> MLPKDKLNPPTPSIYLENKRDAFFPPLHQFCTNPKNPVTVIRG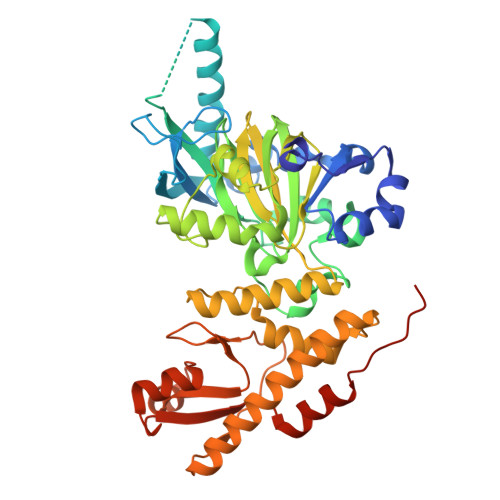LAGALKLDLGLFSTKTLVEANNEHMVEVRTQLLQPADENWDPTGTKKIWRCESNRSHTTIAKYAQYQASSFQESLREENEKRTQHKDHSDNESTSSENSGRRRKGPFKTIKFGTNIDLSDNKKWKLQLHELTKLPAFARVVSAGNLLTHVGHTILGMNTVQLYMKVPGSRTPGHQENNNFCSVNINIGPGDCEWFVVPEDYWGVLNDFCEKNNLNFLMSSWWPNLEDLYEANVPVYRFIQRPGDLVWINAGTVHWVQAVGWCNNIAWNVGPLTACQYKLAVERYEWNKLKSVKSPVPMVHLSWNMARNIKVSDPKLFEMIKYCLLKILKQYQTLREALVAAGKEVIWHGRTNEEPAHYCSICEVEVFNLLFVTNESNTQKTYIVHCHDCARKTSKSLENFVVLEQYKMEDLIQVYDQFTLALSLSSSSAENLYFQ>AFMPDARAYWVTSDLIAWNVGELEAQSVCLYASRAAAMSLSPSNGGIQGYDSKVELQPESAGLPETVTQKFPFISSYRAFRVPSSVDVASLVKCQLVVASFGADGKHVDVTGLQLPGVLDDMFAYTGPLGAVFSEDSVSLHLWAPTAQGVSVCFFDGPAGPALETVQLKESNGVWSVTGPREWENRYYLYEVDVYHPTKAQVLKCLAGDPYARSLSANGARTWLVDINNETLKPASWDELADEKPKLDSFSDITIYELHIRDFSAHDGTVDSDSRGGFRAFAYQASAGMEHLRKLSDAGLTHVHLLPSFHFAGVDDIKSNWKFVDECELATFPPGSDMQQAAVVAIQEEDPYNWGYNPVLWGVPKGSYASDPDGPSRIIEYRQMVQALNRIGLRVVMDVVYNHLDSSGPCGISSVLDKIVPGYYVRRDTNGQIENSAAMNNTASEHFMVDRLIVDDLLNWAVNYKVDGFRFDLMGHIMKRTMMRAKSALQSLTTDAHGVDGSKIYLYGEGWDFAEVARNQRGINGSQLNMSGTGIGSFNDRIRDAINGGNPFGNPLQQG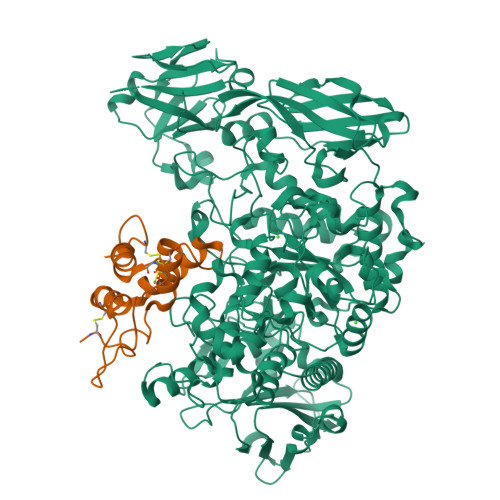FNTGLFLEPNGFYQGNEADTRRSLATYADQIQIGLAGNLRDYVLISHTGEAKKGSEIHTFDGLPVGYTASPIETINYVSAHDNETLFDVISVKTPMILSVDERCRINHLASSMMALSQGIPFFHAGDEILRSKSIDRDSYNSGDWFNKLDFTYETNNWGVGLPPSEKNEDNWPLMKPRLENPSFKPAKGHILAALDSFVDILKIRYSSPLFRLSTANDIKQRVRFHNTGPSLVPGVIVMGIEDARGESPEMAQLDTNFSYVVTVFNVCPHEVSMDIPALASMGFELHPVQVNSSDTLVRKSAYEAATGRFTVPGRTVSVFVEPRC[2x];>[2x]TLESVKDECQPGVDFPHNPLATCHTYVIKRVCGRGPSRPMLVKERCCRELAAVPDHCRCEALRILMDGVRTPEGRVVEGRLGDRRDCPREEQRAFAATLVTAAECNLSSVQEPGHHHHHH>GHMNQFVTNTKNVIRGKYHPEFLQNEVLADIFAHTAQTLPDKTALIEADKTLSYGELYQQALIMAQHLALKGVKPGHIVGLWLPRGIELLKAQLAICLSGAAWLPFDMDTPADRIAVCLEDAEAVGMITTDEWYEHLAEVPQTKWTNTELQKPLSESVSLAKTTPDQPAYIIYTSGSTGKPKGIVITQKNICHFLRSENSILGIQEQDKVYQGFSVAFDMSFEEIWLSYLVGATLWIAPKSLVSDPERLCQTLKQEQITVLHAVPTLLALFPEDVPNLRIINLGGEMCPDSLVDRWALPHHQMFNTYGPTETTVSASLELLERGKPVTIGKPLPNYGMLVINSERELLEQGETGELCIFGPSVAQGYLGRPDLTADKFIENPWAMSVEEELLYRTGDLAKIDEFGQVHCLGRAD[2x]

Here, we report a δ-poly-L-ornithine synthetase from Acinetobacter baumannii, which we name PosA. Nonribosomal peptide synthetase (NRPS) enzymes, usually composed of condensation, adenylation, and thiolation domains, are involved in peptide natural product biosynthesis to produce antibiotics and siderophores. Activity analyses show that the A. baumannii homolog activates L-Orn and the full-length protein produces isopeptide polymers in vitro. Structures of the isolated adenylation domain from PosA are presented with several diamino acids and biochemical assays identify important substrate binding residues.

To better understand the substrate binding in PosA, we solved four structures of the isolated adenylation domain. All four structures were solved in the same space group P212121 with two protomers per asymmetric unit. Data were collected to 2.2–2.5 Å for all four structures and refined to completion through iterative cycles of model building and refinement. The structure of adenylation domain N-terminal subdomain (Acore) shows the typical acyl-CoA synthetase fold with three subdomains. The PosA sequence contains a 16-residue insertion at residue Tyr132 to Glu147 compared to εPL synthetase that results in an extra α-helix and an antiparallel β-strand, located over 20 Å from the active site. The N-terminal adenylation domain of the A. baumannii homolog (residues 1–512) was cloned, expressed in E. coli BL21 (DE3), and purified to homogeneity for enzymatic assay and crystallization. The potential preference of a cationic amino acid substrate was supported by a crystal structure, described below, which confirmed the presence of negatively charged Glu221 and polar residues Thr304 and Ser313 at the side chain binding pocket. Density for both ornithine isomers was unambiguous; the electron density for the lysine ligand was less complete for the carboxylate and amine, suggesting the longer substrate may adopt multiple conformations in the active site of the crystallized protein. For other members of this family of adenylate forming enzymes, including several firefly luciferases21,22 and the free-standing adenylation domains BasE23 and VinN24, only the N-terminal or Acore domain of the adenylation domain was observed in the crystal structures; no density was observed for the C-terminal Asub domain.>TKGLVLGIYSKEKEEDEPQFTSAGENFNKLVSGKLREILNISGPPLKAGKTRTFYGLHEDFPSVVVVGLGKKTAGIDEQENWHEGKENIRAAVAAGCRQIQDLEIPSVEVDPCGDAQAAAEGAVLGLYEYDDLKQKRKVVVSAKLHGSEDQEAWQRGVLFASGQNLARRLMETPANEMTPTKFAEIVEENLKSASIKTDVFIRPKSWIEEQEMGSFLSVAKGSEEPPVFLEIHYKGSPNASEPPLVFVGKGITFDSGGISIKAAANMDLMRADMGGAATICSAIVSAAKLDLPINIVGLAP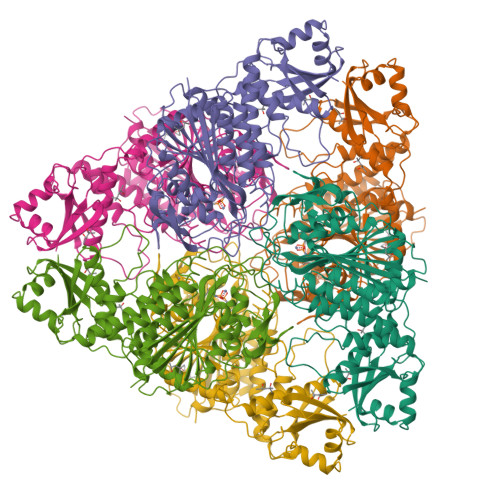LCENMPSGKANKPGDVVRARNGKTIQVDNTDAEGRLILADALCYAHTFNPKVIINAATLTGAMDIALGSGATGVFTNSSWLWNKLFEASIETGDRVWRMPLFEHYTRQVIDCQLADVNNIGKYRSAGACTAAAFLKEFVTHPKWAHLDIAGVMTNKDEVPYLRKGMAGRPTRTLIEFLFRFSQ[2x]>MNNIFDIARMAGVSKTTVSRVINNQPGVREETRIKVQEAIKKLNYVPNHAARSLVSRKSGVIGVVLNEFNASVYLKLANYLEKFAYNYNYNVVFCSSNDNYESKSRYVQYFTGGAADGLILFGSDTRDKELVKRILKTGFPLVLIENYFNDINVNDVIINNFSGAVNAVNYLVGLGHRKIAHITGNVNHRAALERLNGYIRALNENGLAYSKEYVINTDSGEQSGCKAADQLLKLKEPPTAVFTFNDMQGYEVIQRASELGLSVPRDLSVVGFDNIYDIFRFIPSNVRLTSMKQPMEKVAEAAIQLMVANIDNADEQP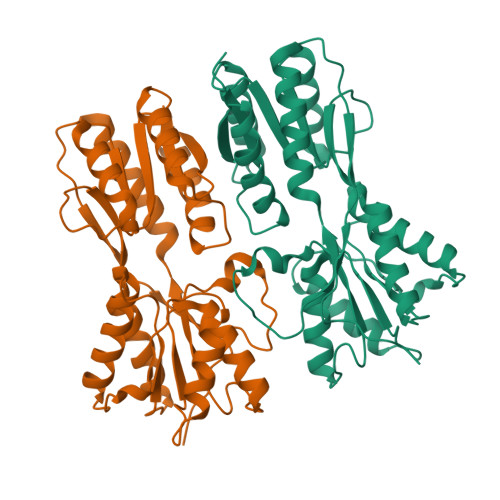KVISFETELFHGTSCCERKHHHHHH[4x]> GPKLKGRKIVGGKAEGEVIVSR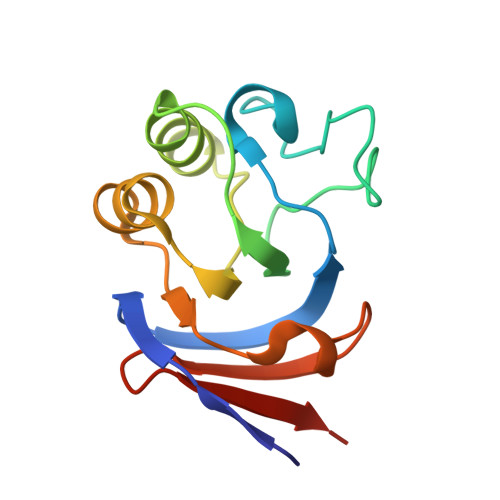KPLSFLGGVDPETGIVTDAESDIRGQSIAGKILVFPRGKGSTVGSYVIYALKKNNKAPKAIIVGEAETIVATGAIISDIPMVDGVDVSKLKTGMKVRVDADSGEVEILEDGE>MMSKEAFFLKQSFHLRLRDDKRIVFSEPAVMGIINVSPNSFYHPHLDLNSALRTAEKMVDEGADILDIGGEATNPFVDIKTDSPSTQIELDRLLPVIDAIKKRFPQLISVDTSRPRVMREAVNTGADMINDQRALQLDDALTTVSALKTPVCLMHFPSETRKPGSTTHFYFLQSVKKE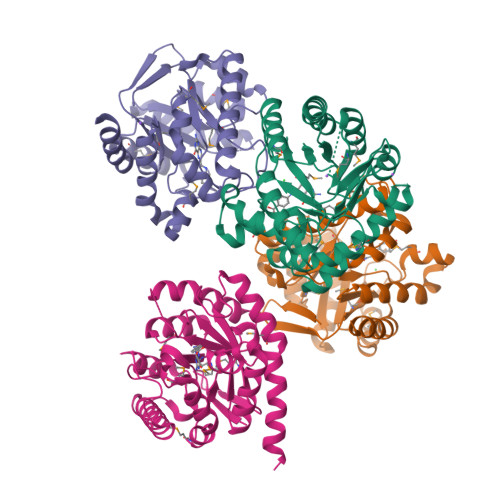LQESIQRCKKAGISEDRIIIDPGFGQGNYGKNVSENFYLLNKLPEFVAMGLPVLSGWSRKSMIGDVLNQPPENRLFGSIAADVLAVYHGASIIRTHDVKATREAIKIATYTRSVDTIEEENLYFQGHHHHHHHHHH[4x]>[2x]MRIAVDAMGGDHAPKAVIDGVIKGIEAFDDLHITLVGDKTTIESHLTTTSDRITVLHADEVIEPTDEPVRAVRRKKNSSMVLMAQEVAENRADACISAGNTGALMTAGLFIVGRIKGIDRPALAPTLPTVSGDGFLLLDVGANVDAKPEH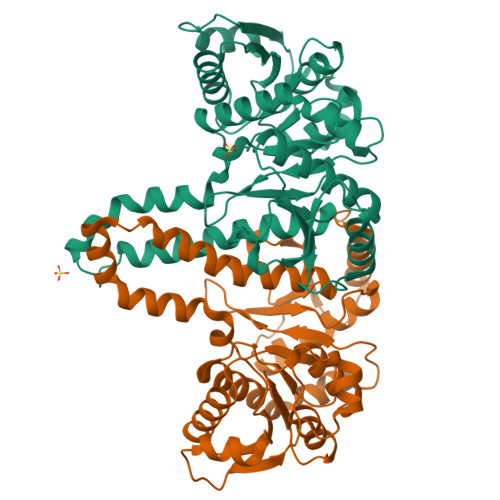LVQYAIMGSVYSQQVRGVTSPRVGLLNVGTEDKKGNELTKQTFQILKETANINFIGNVEARDLLDDVADVVVTDGFTGNVTLKTLEGSALSIFKMMRDVMTSTLTSKLAAAVLKPKLKEMKMKMEYSNYGGASLFGLKAPVIKAHGSSDSNAVFHAIRQAREMVSQNVAALIQEEVLEHHHHHH>MHHHHHHLPNITILATGGDIAGGGDSATKSNYTVGKVGVENLVNAVPQLKDIANVKGEQVVNIGSQDMNDNVWLTLAKKINTDCDKTDGFVITHGVDTMEETAYFLDLTVKCDKPVVMVGAMRPSTSMSADGPFNLYNAVVTAADKASANRGVLVVMNDTVLDGRDVTTTNTTDVATFKSVNYGPLGYIHNGKIDYQRTPARKHTSDTPFDVSKLNELPKVGIVYNYANASDLPAKALVDAGYDGIVSAGVGNGNL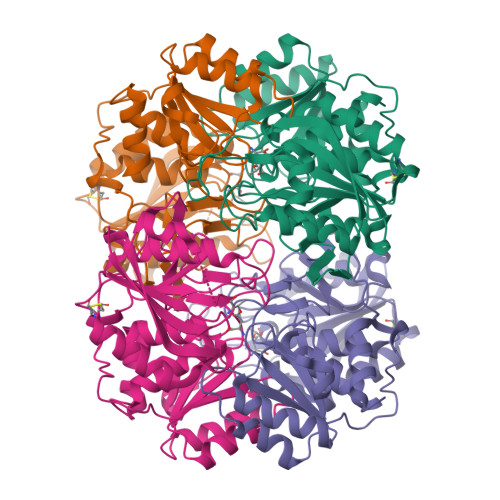YKSVFDTLATAAKTGTAVVRSSRVPTGATTQDAEVDDAKYGFVASGTLNPQKARVLLQLALTQTKDPQQIQQIFNQY[4x]> MSTSTSQIAVEYPIPVYRFIVSVGDEKIPFNSVSGLDISYDTIEYRDGVGNWFKMPGQSQSTN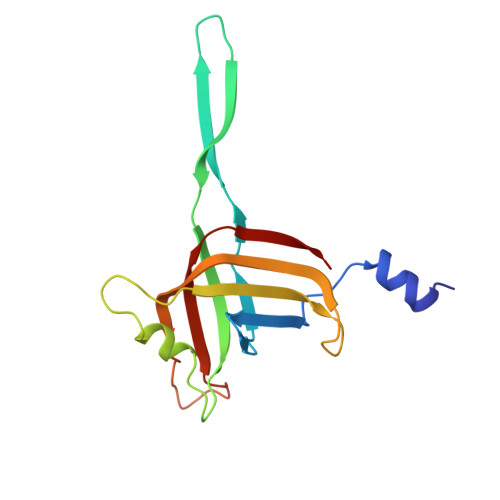ITLRKGVFPGKTELFDWINSIQLNQVEKKDITISLTNDAGTELLMTWNVSNAFPTSLTSPSFDATSNDIAVQEITLMADRVIMQAV> SDEADEAYSVTEQLTMTGINRIRQKINAHGIPVYLCEACGNPIPEAR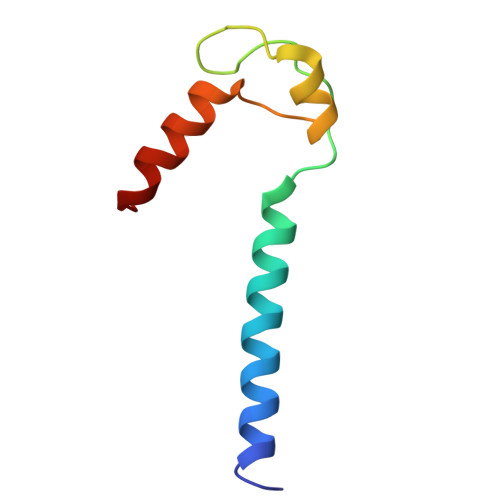RKIFPGVTLCVECQAYQERQRKHYA>QGMQYEWRKAELIGQLLNLGVTPGGVLLVHSSFRSVRPLEDGPLGLIEALRAALGPGGTLVMPSWSGLDDEPFDPATSPVTPDLGVVSDTF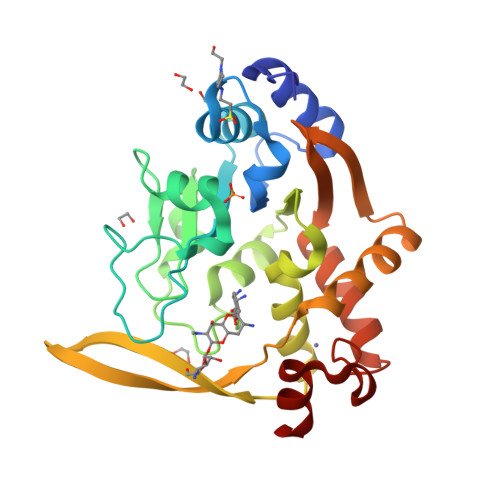WRLPNVKRSAHPFAFAAAGPQAEQIISDPLPLPPHSPASPVARVHELDGQVLLLGVGHDANTTLALAELMAKVPYGVPRHCTILQDGKLVRVDYLENDHCCERFALADRWLKEKSLQKEGPVGHAFARLIRSRDIVATALGQLGRDPLIFLHPPEAGCEECDAARQSIG[6x]>MIVTSGVLVENGKVLLVKHKRLGVYIYPGGHVEHNETPIEAVKREFEEETGIVVEPIGFTYGIIDENAVERPMPLVILEEVVKYPEETHIHFDLIYLVKRVGGDLKNGEWIDVREID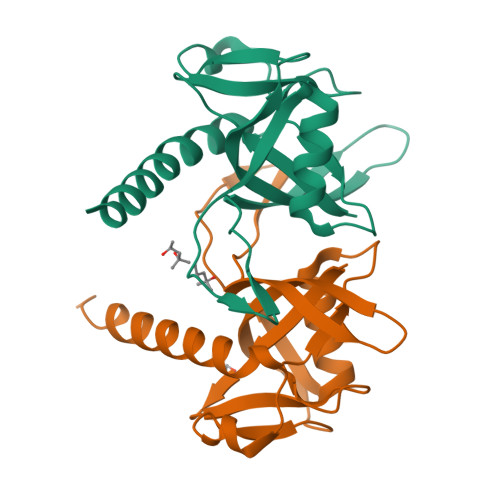RIETFPNVRKVVSLALSTLYRLGKISKLAAALEHHHHHH[4x]> DCPA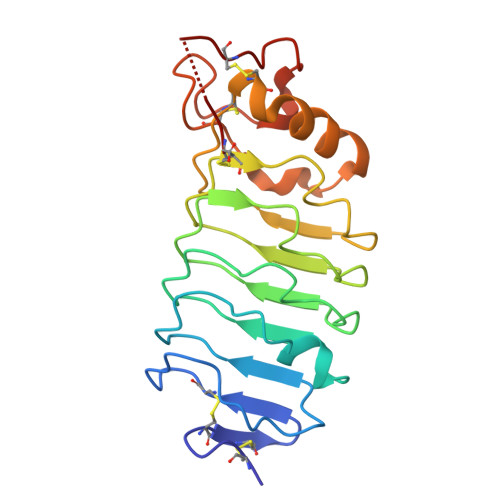MCHCEGTTVDCTGRGLKEIPRDIPLHTTELLLNDNELGRISSDGLFGRLPHLVKLELKRNQLTGIEPNAFEGASHIQELQLGENKIKEISNKMFLGLHQLKTLNLYDNQISCVMPGSFEHLNSLTSLNLASNPFNCNCHLAWFAEWLRKKSLNGGAARCGAPSKVRDVQIKDLPHSEFKCSSENSEGC>MASVVGTPKSAEQIQQEWDTNPRWKDVTRTYSAEDVVALQGSVVEEHTLARRGAEVLWEQLHDLEWVNALGALTGNMAVQQVRAGLKAIYLSGWQVAGDANLSGHTYPDQSLYPANSVPQVVRRINNALQRADQIAKIEGDTSVENWLAPIVADGEAGFGGALNVYELQKALIAAGVAGSHWEDQLASEKKSGHLGGKVLIPTQQHIRTLTSARLAADVADVPTVVIARTDAEAATLITSDVDERDQPFITGERTREGFYRTKNGIEPCIARAKAYAPFADLIWMETGTPDLEAARQFSEAVKAEYPDQMLAYNCSPSFNWKKHLDDATIAKFQK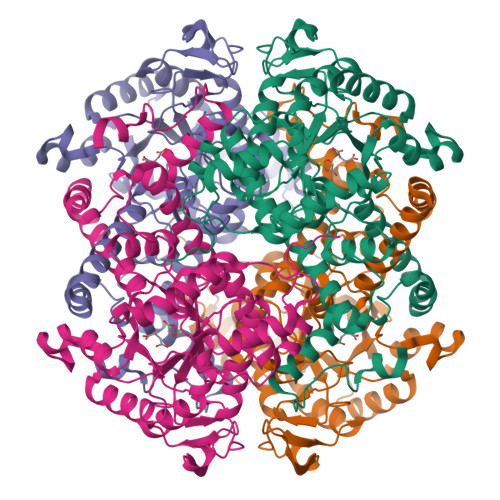ELAAMGFKFQFITLAGFHALNYSMFDLAYGYAQNQMSAYVELQEREFAAEERGYTATKHQREVGAGYFDRIATTVDPNSSTTALTGSTEEGQFH[4x]> APLVHHHHHHALDENLYFQGALADVSRPPHARKTGGSSPETKYDQPPKCDISGKEAISALSRAKSKHCRQEIGETYCRHKLGLLMPEKVTRFCPLEGKANKNVQWDEDSVEYMPANPVRIAFVLVVHGRASRQLQRMFKAIYHKDHFYYIHVDKRSNYLHRQVLQVSRQYSNVRVTPWRMATIWGGASLLSTYLQSMRDLLEMTDWPWDFFINLSAADYPIRTNDQLVAFLSRYRDMNFLKSHGRDNARFIRKQGLDRLFLECDAHMWRLGDRRIPEGIAVDGGSDWFLLNRRFVEYVTFSTDDLVTKMKQFYSYTLLPAESFFHTVLENSPHCDTMVDNNLRITNWNRKLGCKCQYKHIVDWCGCSPNDFKPQDFHRFQQTARPTFFARKFEAVVNQEIIGQLDYYLYGNYPAGTPGLRSYWENVYDEPDGIHSLSDVTLTLYHSFARLGLRRAETSLHTDGENSCRYYPMGHPASVHLYFLADRFQGFLIKHHATNLAVSKLETLETWVMPKKVFKIASPPSDFGRLQFSEVGTDWDAKERLFRNFGGLLGPMDEPVGMQKWGKGPNVTVTVIWVDPVNVIAATYDILIESTAEFTHYKPPLNLPLRPGVWTVKILHHWVPVAETKFLVAPLTFSNRQPIKPEEALKLHNGPLRNAYMEQSFQSLNPVLSLPINPAQVEQARRNAASTGTALEGWLDSLVGGMWTAMDICATGPTACPVMQTCSQTAWSSFSPDPKSELGAVKPDGRLR;> QEEEYSGGGQGG

The first enzyme in the pathway, peptide O-xylosyltransferase (XT, EC 2.4.2.26), catalyzes the transfer of xylose from uridine diphosphate (UDP)-α-D-xylose onto serine and thus determines the site(s) of GAG attachment on the core protein. XT1 and XT2 are type II transmembrane proteins consisting of a short amino-terminal region facing the cytosol, a single transmembrane helix, a stem region required for Golgi localization (Schön et al., 2006), a catalytic GT-A domain (Lairson et al., 2008, Müller et al., 2006), and a unique C-terminal domain of unknown function, termed “Xylo_C” in the Pfam database (Finn et al., 2008). XT1 has a two-lobed structure, with one lobe comprising the catalytic GT-A domain and the other comprising the Xylo_C domain. To better understand the initial step of GAG biosynthesis, we have determined crystal structures of human XT1 complexed with UDP-xylose and various PG-derived acceptor peptides.

To visualize how the different amino acid substitutions are accommodated in the peptide binding cleft, we selected five variants of the bikunin-derived peptide for structure analysis (peptides 3–7). In contrast, position −1 has a wide tolerance for uncharged amino acids, accommodating even large aromatic residues such as tryptophan. The substitution of glycine by tyrosine at position −1 (peptide 4) causes a similar widening of the peptide binding cleft. The tyrosine side chain packs against the side chain of F498, displacing it by ∼1 Å. This is accompanied by a flip of the peptide bond between positions −1 and −2 of the acceptor peptide, which, however, does not affect the conformation of the glutamic acid side chain at position −2.>MSLIYEDLVKSLDSKQQAYVDLKLPDPTNGEFLLAVFHMIPGGDLNVLQAAAEIAAESSTGTNIKVSTETAFSRTMNARVYQLDLERELVWIAYPWRLFDRGGNVQNILTYIIGNILGMKEIQALKLMDIWFPPSMLEQYDGPSYTVDDMRKYLDVYDRPILGTIVKPKMGLTSAEYAEVCYDFWVGGGDFVKNDEPQANQDFCPYEKMVAHVKEAMDKAVKETGQKKVHSFNVSAADFDTMIERCEMITNAGFEPGSYAFLIDGITAGWMAVQTLRRRYPDVFLHFHRAAHGAFTRQENPIGFSVLVLSKFARLAGASGIHTGTAGIGKMKGTPAEDVVAAHSIQYLKSPGHFFEQTWSKIMDTDKDVINLVNEDLAHHVILEDDSWRAMKKCCPIVSGGLNPVKLKPFIDVMENVDFITTMGSGVHSHPGGTQSGAKALVQACDAYLQGMDIEEYAKDHKELAEAIEFYLNR[5x]

Ribulose-1,5-bisphosphate (RuBP)2 carboxylase/oxygenase (Rubisco) catalyzes the carboxylation of RuBP to yield two molecules of 3-phosphoglycerate (3-PGA). The Rubisco from the Antarctic-dwelling methanogenic archaeon Methanococcoides burtonii likely acts as part of the AMP/ADP-recycling pathway by scavenging the RuBP by-product. Five L2 dimers assemble into a rare (L2)5 structure observed exclusively in thermostable archaeal Rubiscos. MbR contains a unique 26–30-amino acid insertion between α6 and β7 at the bottom of the βα-barrel, and deleting this “bonus” sequence yields enzymes that are catalytically competent, albeit with altered kinetic properties, and are incapable of assembling into (L2)5 enzymes.

The MbR asymmetric unit contains five LSus. Applying the crystallographic symmetry results in the L10 biological unit consistent with previous biochemical observations. The MbR structure (half of the biological unit) contains 10 Mg2+ ions, 5 Cl− ions, and 294 water molecules. As expected, Mg2+ binds to the active site (5 per half-L10 decamer), stabilizing the carbamate formed at the active site lysine. The Mg2+ ion that stabilizes the carbamylated catalytic Lys-193 coordinates to O2, O3, and O6 of 2-CABP upon substrate binding. A second binding site for Mg2+ was also inferred from difference electron density at the interface of the L2 dimers (two Mg2+ per interface and 5 per half-L10 decamer). This Mg2+ ion is coordinated by a structural motif unique to MbR, which adopts a loop-helix-loop conformation. The motif, which forms a separate domain, is encoded by a C-terminal 29-amino acid insertion in MbR (residues 361–389) and corresponds to a β-hairpin motif predicted from sequence data. Although the search model was at the lower size limit for the Dali server, these results suggest that the structure of this motif is unique. Because of its strategic location and its clear functional role (see below), we named it the Rubisco assembly domain (RAD). The Mg2+ ion is ligated by oxygen donor atoms provided by the side chains of Asp-366 and Asp-368 located at the N-terminal end of the RAD helix αJ and Glu-179 and Asp-183 located in helix α1 of the βα-barrel in the LSu of the neighboring L2 dimer.> MGSAEIQPRSDEKRILSNVAVLEGAPPLSEHWQLFNNNEVLFNEARTAQAATVVFSLQQNAQIEPLARSIHTLRRQRGSAMKILVRENTASLRATDERLLLACGANMVIPWNAPLSRCLTMIESVQGQKFSRYVPEDITTLLSMTQPLKLRGFQKWDVFCNAVNNMMNNPLLPAHGKGVLVALRPVPGIRVEQALTLCRPNRTGDIMTIGGNRLVLFLSFCRIND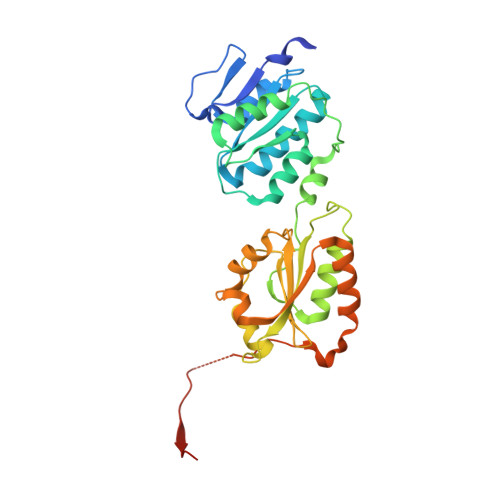LDTALNHIFPLPTGDIFSNRMVWFEDDQISAELVQMRLLAPEQWGMPLPLTQSSKPVINAEHDGRHWRRIPEPMRLLDDAVERSS> GSPHMDEISETNTIFKLEGVSVLSPLRKKLDLVFYLSNVDGSPVITLLKGNDRELSIYQLNKNIKMASFLPVPEKPNLIYLFMTYTSCEDNKFSEPVVMTLNKENTLNQFKNLGLLDSNVTDFEKCVEYIRKQAILTGFKISNPFVNSTLVDTDAEKINSFHLQCHRGTKEGTLYFLPDHIIFGFKKPILLFDASDIESITYSSITRLTFNASLVTKDGEKYEFSMTDQTEYAKIDDYVKRKQMKDKSMSEE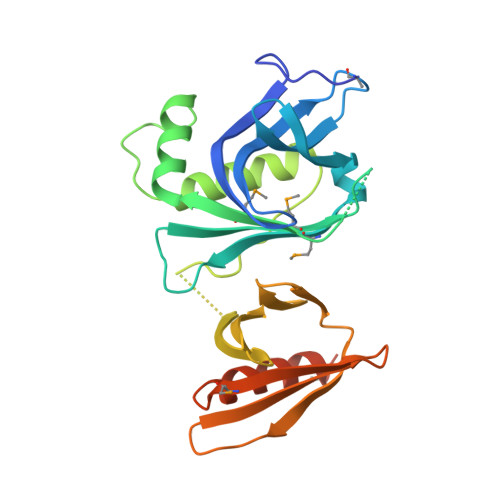LKAKSKSKG> 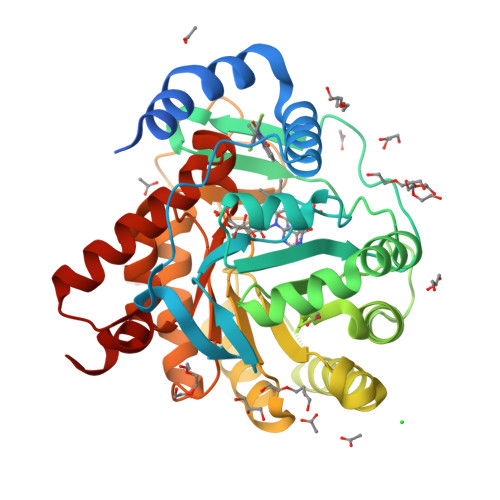MAWRHLKKRAQDAVIILGGGGLLFASYLMATGDERFYAEHLMPTLQGLLDPESAHRLAVRFTSLGLLPRARFQDSDMLEVRVLGHKFRNPVGIAAGFDKHGEAVDGLYKMGFGFVEIGSVTPKPQEGNPRPRVFRLPEDQAVINRYGFNSHGLSVVEHRLRARQQKQAKLTEDGLPLGVNLGKNKTSVDAAEDYAEGVRVLGPLADYLVVNVSSPNTAGLRSLQGKAELRRLLTKVLQERDGLRRVHRPAVLVKIAPDLTSQDKEDIASVVKELGIDGLIVTNTTVSRPAGLQGALRSETGGLSGKPLRDLSTQTIREMYALTQGRVPIIGVGGVSSGQDALEKIRAGASLVQLYTALTFWGPPVVGKVKRELEALLKEQGFGGVTDAIGADHRR> MGIDINTKIFNSVAEVFQKAQGSYAGHRKHIAVLKKIQSKAVEQGYEDAFNFWFDKLVTKILPLKKNEIIGDRIVKLVAAFIASLERELILAKKQNYKLTNDEEGIFSRFVDQFIRHVLRGVESPDKNVRFRVLQLLAVIM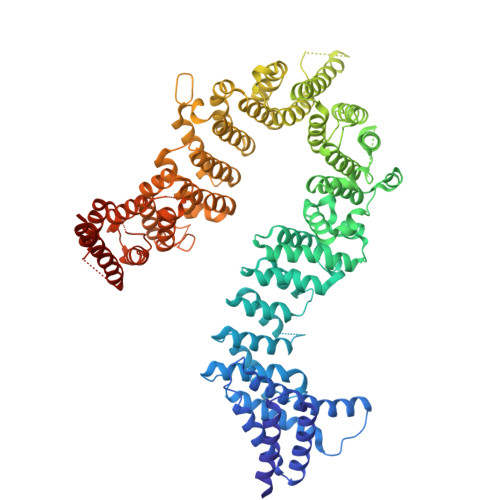DNIGEIDESLFNLLILSLNKRIYDREPTVRIQAVFCLTKFQDEEQTEHLTELSDNEENFEATRTLVASIQNDPSAEVRRAAMLNLINDNNTRPYILERARDVNIVNRRLVYSRILKSMGRKCFDDIEPHIFDQLIEWGLEDRELSVRNACKRLIAHDWLNALDGDLIELLEKLDVSRSSVCVKAIEALFQSRPDILSKIKFPESIWKDFTVEIAFLFRAIYLYCLDNNITEMLEENFPEASKLSEHLNHYILLRYHHNDISNDSQSHFDYNTLEFIIEQLSIAAERYDYSDEVGRRSMLTVVRNMLALTTLSEPLIKIGIRVMKSLSINEKDFVTMAIEIINDIRDDDIEKQESESDIINNLPPEKEASSATIVLCLTRSSYMLELVNTPLTENILIASLMDTLITPAVRNTAPNIRELGVKNLGLCCLLDVKLAIDNMYILGMCVSKGNASLKYIALQVIVDIFSVHGNTVVDGEGKVDSISLHKIFYKVLKNNGLPECQVIAAEGLCKLFLADVFTDDDLFETLVLSYFSPINSSNEALVQAFAFCIPVYCFSHPAHQQRMSRTAADILLRLCVLWDDLQSSVIPEVDREAMLKPNIIFQQLLFWTDPRNLVNQTGSTKKDTVQLTFLIDVLKIYAQIEKKEIKKMIITNINAIFLSSEQDYSTLKELLEYSDDIAENDNLDNVSKNALDKLRNNLNSLIEEINERSETQTKDENNTANDQYSSILGN> MKIFFITSNPGKVREVANFLGTFGIEIVQLKHEYPEIQAEKLEDVVDFGISWLKGKVPEPFMIEDSGLFIESLKGFPGVYSSYVYRTIGLEGILKLMEGAEDRRAYFKSVIGFYIDGKAYKFSGVTWGRISNEKRGTHGFGYDPIFIPEGSQKTFAEMTIEEKNALSHRGKALKAF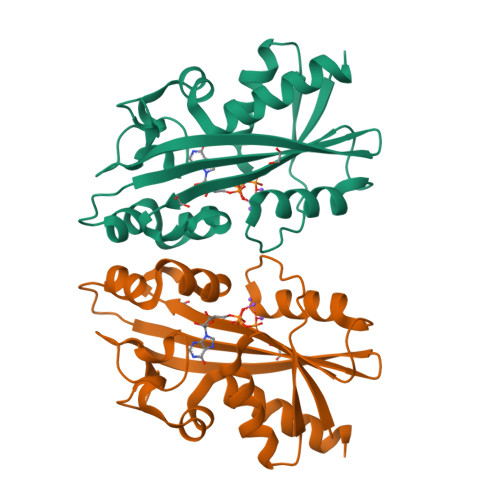FEWLKVNLKY> ASDTAVSNVVNYSTDVIYQIVTDRFVDGNTSNNPTGDLYDPTHTSLKKYFGGDWQGIINKINDGYLTGMGVTAIWISQPVENIYAVLPDSTFGGSTSYHGYWARDFKRTNPYFGSFTDFQNLINTAHAHNIKVIIDFAPNHTSPASETDPTYAENGRLYDNGTLLGGYTNDTNGYFHHYGGTDFSSYEDGIYRNLFDLADLNQQNSTIDSYLKSAIKVWLDMGIDGIRLDAVKHMPFGWQKNFMDSILSYRPVFTFGEWFLGTNEIDVNNTYFANESGMSLLDFRFSQKVRQVFRDNTDTMYGLDSMIQSTASDYNFINDMVTFIDNHDMDRFYNGGSTRPVEQALAFTLTSRGVPAIYYGTEQYMTGNGDPYNRAMMTSFNTSTTAYNVIKKLAPLRKSNPAIAYGTTQQRWINNDVYIYERKFGNNVALVAINRNLSTSYNITGLYTALPAGTYT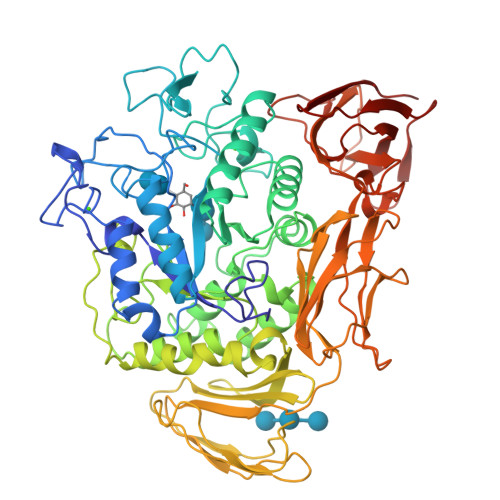DVLGGLLNGNSISVASDGSVTPFTLSAGEVAVWQYVSSSNSPLIGHVGPTMTKAGQTITIDGRGFGTTSGQVLFGSTAGTIVSWDDTEVKVKVPSVTPGKYNISLKTSSGATSNTYNNINILTGNQICVRFVVNNASTVYGENVYLTGNVAELGNWDTSKAIGPMFNQVVYQYPTWYYDVSVPAGTTIQFKFIKKNGNTITWEGGSNHTYTVPSSSTGTVIVNWQQ> ACPAPPPGQPDIRAIGYYTDKAGSVIDPALQQQNKDATAPLDRYAADVARMSDDYLRNGDPAAAQCTLSWLGAWADDGAMLGQMIRVNNDQSFYMRQWMLDAVAMAYLKVHDQANPQQRARIDPWLQKLARANLAYWDN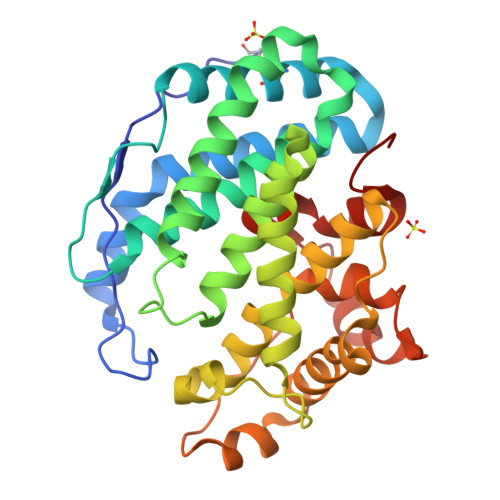PKRRRNNHYYWGGLGVLATGLATDDDALWQAGHAAFQKGIDDIQDDGSLPLEMARGQRALHYHDYALAPLVMMAELARLRGQDWYASRNHAIDRLARRVIEGSRDPAWFNQHTGAAQLPLQASGWVEFYRLRSPDGGVFDAAHARGPFHSPRLGGDLTLMATHGIVRTPL>MNPIHDRTSDYHKYLKVKQGDSDLFKLTVSDKRYIWYNPDPDERDSYECGEIVSETSDSFTFKTVDGQDRQVKKDDANQRNPIKFDGVEDMSELSYLNEPAVFHNLRVRYNQDLIYTYSGLFLVAVNPFKRIPIYTQEMVDIFKGRRRNEVAPHIFAISDVAYRSMLDDRQNQSLLITGESGAGKTENTKKVIQYLASVAGRNQANGSGVLEQQILQANPILEAFGNAKTTRNNNSSEFGKFIEIQFNNAGFISGASIQSYLLEKSRVVFQSETERNYHIFYQLLAGATAEEKKALHLAGPESFNYLNQSGCVDIKGVSDEDEFKITRQAMDIVGFSQEEQMSIFKIIAGILHLGNIKFEKGAGEGAVLKDKTALNAASTVFGVNPSVLEKALMEPRILAGRDLVAQHLNVEKSSSSRDALVKALYGRLFLWLVKKINNVLCSERKAYFIGVLDISGFEIFKVNSFEQLCINYTNEKLQQFFNHHMFKVEQEEYLKEKINWTFIDFGLDSQATIDLIDGRQPPGILALLDEQSVFPNATDNTLITKLHSHFSKKNAKYE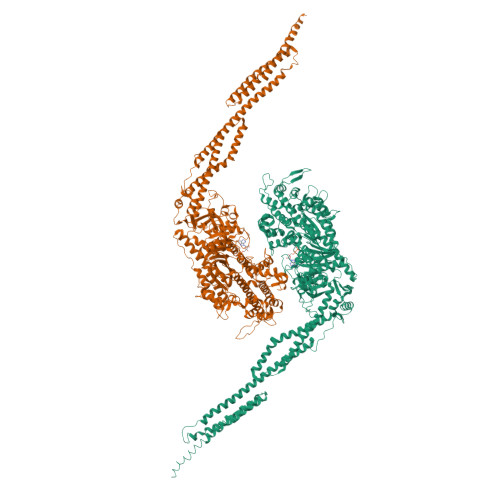EPRFSKTEFGVTHYAGQVMYEIQDWLEKNKDPLQQDLELCFKDSSDNVVTKLFNDPNIASRAKKGANFITVAAQYKEQLASLMATLETTNPHFVRCIIPNNKQLPAKLEDKVVLDQLRCNGVLEGIRITRKGFPNRIIYADFVKRYYLLAPNVPRDAEDSQKATDAVLKHLNIDPEQYRFGITKIFFRAGQLARIEEAREQRLGSEQTKSDYLKRANELVQWINDKQASLESRDFGDSIESVQSFMNAHKEYKKTEKPPKGQEVSELEAIYNSLQTKLRLIKREPFVAPAGLTPNEIDSTWSALEKAEQEHAEALRIELKRQKKIAVLLQKYNRILKKLENWATTKSVYLGSNETGDSITAVQAKLKNLEAFDGECQSLEGQSNSDLLSILAQLTELNYNGVPELTERKDTFFAQQWTGVKSSAETYKNTLLAELERLQKIEDLHHHHHHH[2x]N6-(buta-2,3-dienyl)adenine 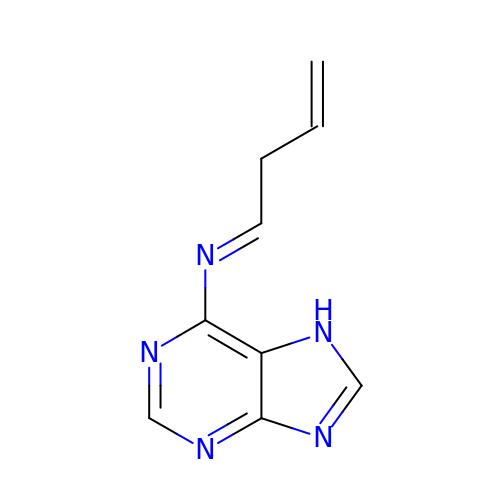| C9 H9 N5 | FOLHQMCIMSOVSL-ONNFQVAWSA-N>GRPVLYQVVAQHSYSAQGPEDLGFRQGDTVDVLCEVDQAWLEGHCDGRIGIFP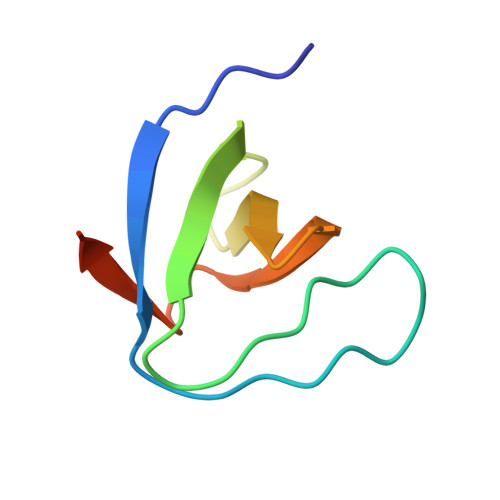KCFVVPAGPRMS[2x]>GSQKERLLDELTLEGVARYMQSERCRRVICLVGAGISTSAGIPDFRSPSTGLYDNLEKYHLPYPEAIFEISYFKKHPEPFFALAKELYPGQF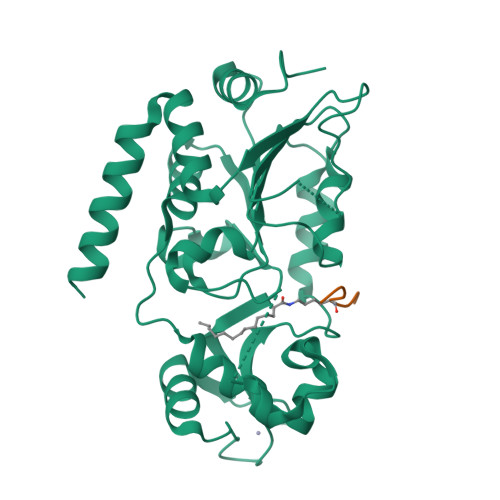KPTICHYFMRLLKDKGLLLRCYTQNIDTLERIAGLEQEDLVEAHGTFYTSHCVSASCRHEYPLSWMKEKIFSEVTPKCEDCQSLVKPDIVFFGESLPARFFSCMQSDFLKVDLLLVMGTSLQVQPFASLISKAPLSTPRLLINKEKAGGGGMDFDSKKAYRDVAWLGECDQGCLALAELLGWKKELEDLVRREHASIDAQS[2x];>LPKXTGG[2x]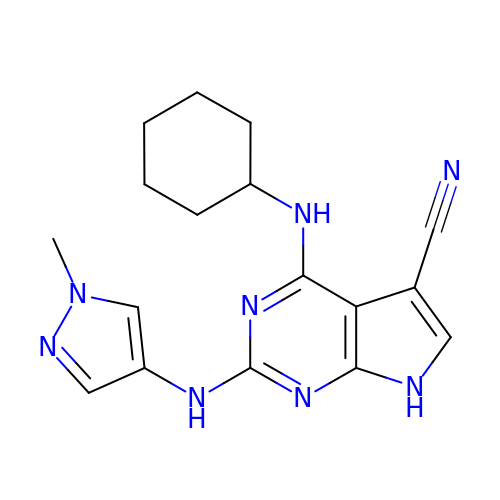4-(cyclohexylamino)-2-[(1-methylpyrazol-4-yl)amino]-7H-pyrrolo[2,3-d]pyrimidine-5-carbonitrile | C17 H20 N8 | KGMINTBDNKGRFK-UHFFFAOYSA-N> MACNFQFPEIAYPGKLICPQYGTENKDGEDIIFNYVPGPG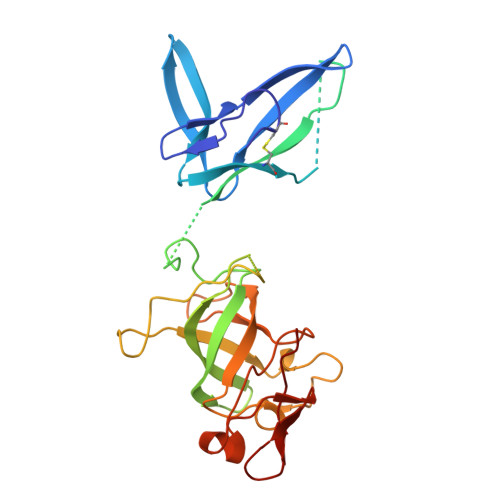TKLIQYEHNGRTLEAITATLVGTVRCEEEKKTDQEEEREGTDQSTEEEKSVDASPNDVTRRTVKNILVSVLPGTEKGRKTNKYANNDFANNLPKEGDIVLTRVTRLSLQRANVEILAVEDKPSPIDSGIGSNGSGIVAAGGGSGAATFSVSQASSDLGETFRGIIRSQDVRSTDRDRVKVIECFKPGDIVRAQVLSLGDGTNYYLTTARNDLGVVFARAANGAGGLMYATDWQMMTSPVTGATEKRKCAKPF ME-A-9-N-(NAPHTHYL-2-CARBONYL)-AMINO-9-DEOXY-NEU5AC | C23 H28 N2 O9 | 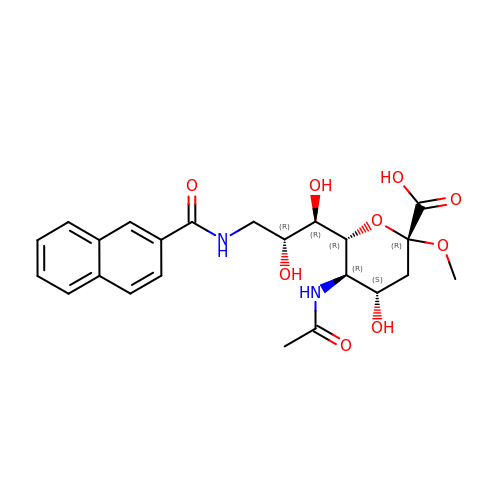NCJJDBXUFQPTHE-GCIBVHORSA-N7-{[(CYCLOHEXYLAMINO)CARBONYL]AMINO}HEPTANOIC ACID | C14 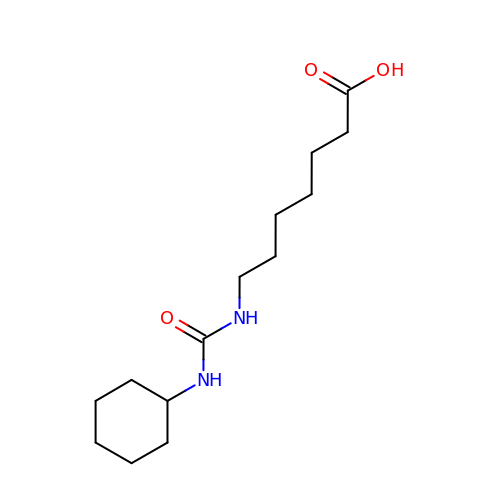H26 N2 O3 | GYTIWWDVOFXKPF-UHFFFAOYSA-N> GSPRTVEEIFKDYSARRAALLRALTKDVDDFYSQCDPEKENLCLYGHPNESWEVNLPAEEVPPELPEPALGINFARDGM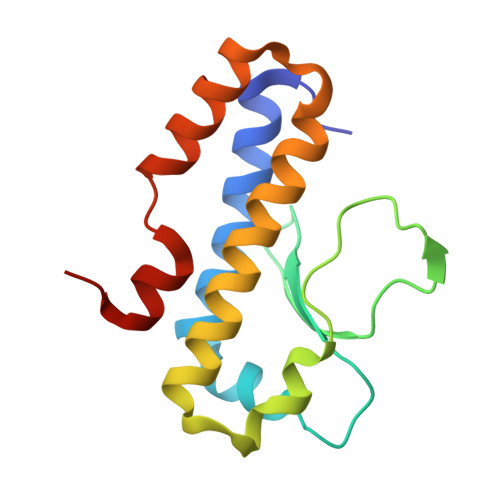QRKDWLSLVAVHSDCWLLSVSFYFGARLNRNERKRLFSLINDLPTLFDVVTGRKAM> TFKSAVKALFDYKAQREDELTFTKSAIIQNVEKQDGGWWRGDYGGKKQLWFPSNYVEEM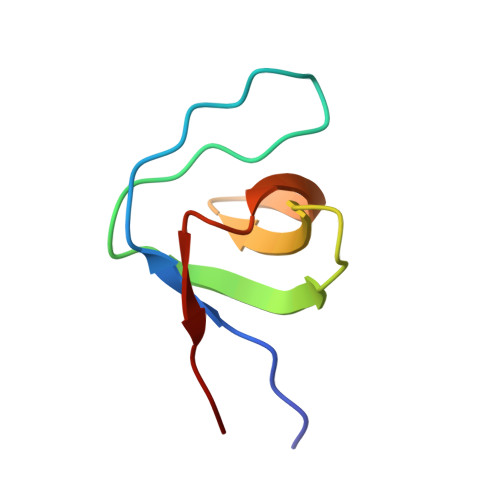IN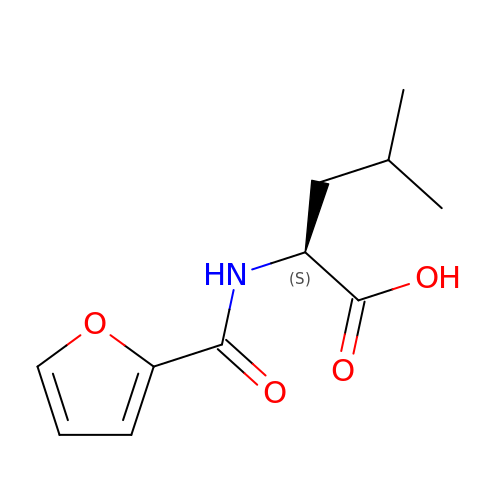FUROYL-LEUCINE | C11 H15 N O4 | LXBURZIESWDWIV-QMMMGPOBSA-N> MHHHHHHLVPRGSPSPPGNLRVTDVTSTSVTLSWEPPPGPITGYRVEYREAGGEWKEVTVPGSETSYTVTG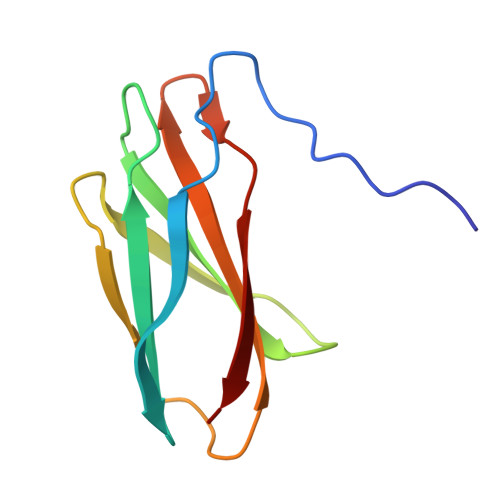LKPGTEYEFRVRAVNGAGEGPPSSVSVTT> MPFEIVFEGAKEFAQLIDTASKLIDE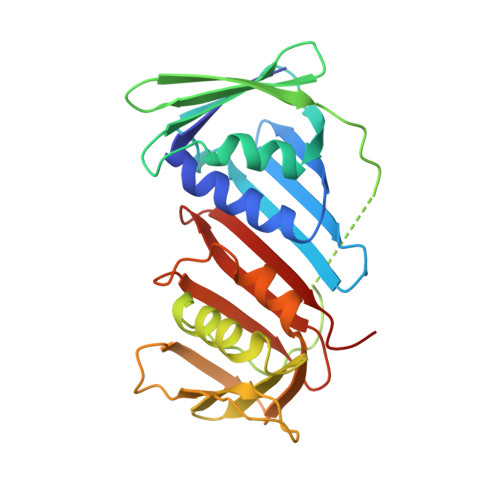AAFKVTEDGISMRAMDPSRVVLIDLNLPSSIFSKYEVVEPETIGVNLDHLKKILKRGKAKDTLILKKGEENFLEITIQGTATRTFRVPLIDVEEMEVDLPELPFTAKVVVLGEVLKAAVKDASLVSDSIKFIARENEFIMKAEGETQEVEIKLTLEDEGLLDIEVQEETKSAYGVSYLSDMVKGLGKADEVTIKFGNEMPMQMEYYIRDEGRLTFLLAPRVEE> MRVLVTGGSGYIGSHTCVQLLQNGHDVIILDNLCNSKRSVLPVIERLGGKHPTFVEGDIR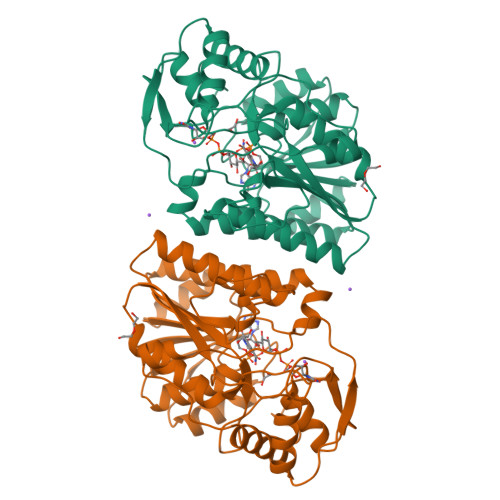NEALMTEILHDHAIDTVIHFAGLKAVGESVQKPLEYYDNNVNGTLRLISAMRAANVKNFIFSSSATVYGDQPKIPYVESFPTGTPQSPFGKSKLMVEQILTDLQKAQPDWSIALLRYFNPVGAHPSGDMGEDPQGIPNNLMPYIAQVAVGRRDSLAIFGNDYPTEDGTGVRDYIHVMDLADGHVVAMEKLANKPGVHIYNLGAGVGNSVLDVVNAFSKACGKPVNYHFAPRREGDLPAYWADASKADRELNWRVTRTLDEMAQDTWHWQSRHPQGYPD>[6x]CGCGAAN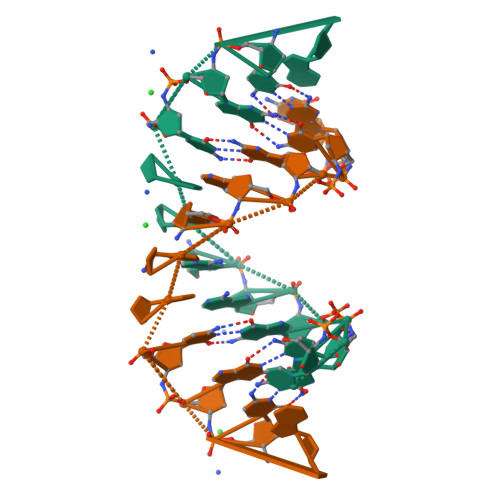NCGCG> MAFARGGLAQTASQTTSSPVRVGLSVDASALGHTIPPDYTGLSYEQAQMANPNYFSGANTQLAGFLRTLGRQGVLRIGGNTSEYTFWNRHAKPTAADEHLAAGPDKGHHAAAREVITPEAVNNLSEFLDKTGWKLIYGLNLGKGTPENAADEAAYVMETIGADRLLAFQLGNEPDLFYRNGIRPASYDFAAYAGDWQRFFTAIRKRVPNAPFAGPDTAYNTKWLVPFADKFKHDVKFISSHYYAEGPPTDPSMTIERLMKPNPRLLGETAGLKQVEADTGLPFRLTETNSCYQGGKQGVSDTFAAALWAGDLMYQQAAAGSTGINFHGGGYGWYTPVAGTPEDGFIARPEYYGMLLFAQAGAGQLLGAKLTDNSAAPLLTAYALRGTDGRTRIALFNKNLDADVEVAISGVASPSGTVLRLEAPRADDTTDVTFGGAPVGASGSWSPLVQEYVPGHSGQFVLHMRKASGALLEFA

Siastatin B is a potent and effective iminosugar inhibitor of three diverse glycosidase classes, namely, sialidases, β-d-glucuronidases, and N-acetyl-glucosaminidases. Surprisingly, siastatin B also inhibits both β-glucuronidases and human heparanase, which cleave β-glucuronic acid residues but not sialic acid or N-acetylated sugars. Herein, we show through crystallographic analysis of protein-inhibitor complexes that siastatin B generates both a hemiaminal and a 3-geminal diol iminosugar (3-GDI) that are, rather than the parent compound, directly responsible for enzyme inhibition. Notably, 3-GDIs are a new class of iminosugar glycoside hydrolase inhibitor, that have been shown to inhibit both GH2 and GH79 β-glucuronidases.

To examine the structural basis for inhibition by our panel of synthetic gluco- and galacto-configured iminosugars, we determined cocrystal structures of the 3-GDIs and either HPSE or AcGH79. Crystal structures with 8 and 9 bound to AcGH79 show that both of these inhibitors are situated in the same binding pocket as that of the galacturonic-noeuromycin 4. Within the iminosugar ring, there is very little conformational change between 8 and 9, and both maintain the 4C1 ring conformation seen for 4. Furthermore, the axial 4-OH present in 8 forms the same H-bond interactions with the protein backbone (with the carbonyl of Asp105) as seen for 4; however, it also has an additional H-bond to an active site water, see Figure 4. The axial 3-OH of geminal diol inhibitors 8 and 9 is found within hydrogen bonding distance of the catalytic nucleophile in both structures. The axial 3-OH is also within 3.0 Å of the εN of His327 in both structures; however, it is unlikely that there is a genuine 3ax-HO···H-εN H-bond interaction as the 3ax-OH is oriented approximately 80° to the plane of the histidine–rather than being in line with the plane, as would be expected. Furthermore, the εN of His327 forms an H-bond, at the appropriate angle, with Glu45. The galacto-configured 3-GDI 8—the breakdown product observed in the active site of HPSE—inhibited AcGH79 (Ki = 5.8 ± 0.5 μM) more potently than did EcGusB (Ki = 137 ± 3 μM). Synthesis of 3-GDIs and their 3-hydroxy counterparts allowed us to dissect the mechanism of their inhibition both kinetically and structurally. These 3-GDIs are well accommodated within the active site pocket and form an additional H-bond interaction with the catalytic nucleophile.4-azido-~{N}-[3,3,3-tris(fluoranyl)propyl]benzamide 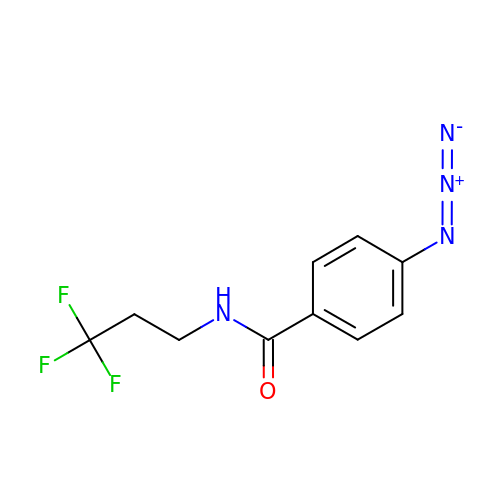| C10 H9 F3 N4 O | PCHDVKCHSJFSLZ-UHFFFAOYSA-N>[4x]MESVERKSESSYLGMRNMQPEQRLSLDPPRLRSTPQDELHDLLCVGFGPASLAIAIALHDALDPRLNKSASNIHAQPKICFLERQKQFAWHSGMLVPGSKAQISFIKDLATLRDPRSSFTFLNYLHQKGRLIHFTNLSTFLPARLEFEDYMRWCAQQFSDVVAYGEEVVEVIPGKSDPSSSVVDFFTVRSRNVETGEISARRTRKVVIAIGGTAKMPSGLPQDPRIIHSSKYCTTLPALLK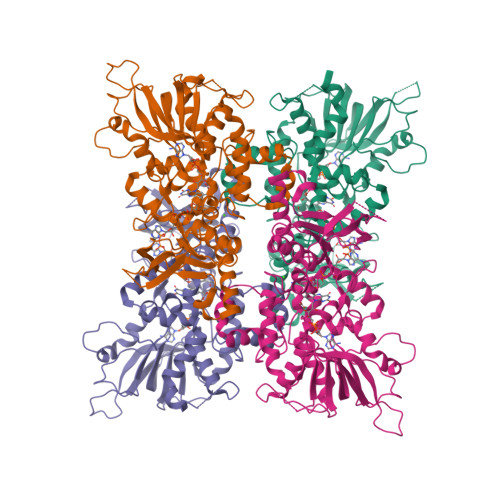DKSKPYNIAVLGSGQSAAEIFHDLQKRYPNSRTTLIMRDSAMRPSDDSPFVNEIFNPERVDKFYSQSAAERQRSLLADKATNYSVVRLELIEEIYNDMYLQRVKNPDETQWQHRILPERKITRVEHHGPQSRMRIHLKSSKPESEGAANDVKETLEVDALMVATGYNRNAHERLLSKVQHLRPTGQDQWKPHRDYRVEMDPSKVSSEAGIWLQGCNERTHGLSDSLLSVLAVRGGEMVQSIFGEQLERAAVQGHQLRAML> MNGIYIWKIGNFGMHLKCQEEEKPVVIHSPGFYTGKPGYKLCMRLHLQLPTAQRCANYISLFVHTMQGEYDS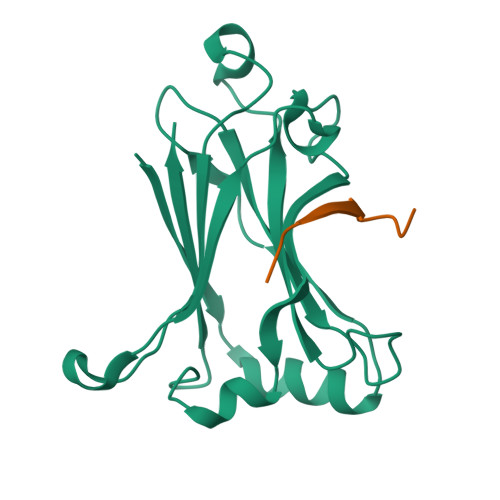HLPWPFQGTIRLTILDQSEAPVRQNHEEIMDAKPELLAFQRPTIPRNPKGFGYVTFMHLEALRQRTFIKDDTLLVRCEVSTLEHHHHHH;> SSQSSSPTEMDENES>MGNIMSASFAPECTDLKTKYDSCFNEWYSEKFLKGKSVENECSKQWYAYTTCVNAALVKQGIKPALDEAREEAPFENGGKL[8x];>MGSSHHHHHHSQDPMVLLHKSTHIFPTDFASVSRAFFNRYPNPYSPHVLSIDTISRNVDQEGNLRTTRLLKKSGKLPTWVKPFLRGITETWIIEVSVVNPANSTMKTYTRNLDHTGIMKVEEYTTYQFDSATSSTIADSRVKFSSGFNMGIKSKVEDWSRTKFDENVKKSRMGMAFVIQKLEEA[8x]

Recently, Ups1, a yeast member of the conserved mitochondrial intermembrane space (IMS) proteins, was shown to mediate PA transfer between the mitochondrial OM and IM in cooperation with Mdm35. Mdm35, another conserved yeast IMS protein, is a binding partner of Ups proteins, and facilitate their import into mitochondria. Surprisingly, two distinct polypeptides of Ups1 and Mdm35 form a single compact domain, the Ups1 part of which corresponds to the START (StAR-related lipid-transfer) domain, likely functioning as a lipid-binding domain. Like other START domain-containing proteins, the Ups1–Mdm35 complex contains a deep pocket that can accommodate a lipid molecule and an Ω-loop likely functioning as a lid for the pocket.

Although we could not obtain good diffraction data of the Ups1–Mdm35 complex with POPA suitable for high-resolution structure determination, we successfully determined the crystal structure of the Ups1–Mdm35 complex with DLPA at 3.20 Å resolution by the molecular replacement method with the Ups1–Mdm35 apo-complex as a search model. The crystallographic asymmetric unit contained eight Ups1–Mdm35 molecules, and two of the eight Ups1–Mdm35 molecules contained a DLPA molecule in the pocket while clear electron density was not observed in the pocket of the remaining six Ups1–Mdm35 molecules. Structural comparison of the Ups1–Mdm35 complexes with and without a bound PA molecule shows the r.m.s. differences of 1.2 and 0.6 Å for 169 Cα atoms of Ups1 and 73 Cα atoms of Mdm35, respectively, indicating that no significant conformational change occurs in Ups1–Mdm35 on PA binding. Interestingly, some of the Ups1–Mdm35 molecules without clear electron density of DLPA in the crystallographic asymmetric unit had the Ω1 lid swung away from the pocket. The bound DLPA molecule is completely enclosed in the pocket of Ups1, with the phosphate head positioned at the bottom of the pocket and the acyl-chain tails oriented toward the entrance of the pocket, yet leaving some empty space in the pocket. At the bottom of the pocket, the positively charged side chains of Arg25 and Lys58 are close to the negatively charged phosphate group of DLPA, and side chains of Tyr26, His33 and Lys58 are within the distance that allows formation of hydrogen bonds with the phosphate oxygen atoms. The hydrophobic acyl-chain tails are in contact with hydrophobic side chains of Thr76, Ile78, Met104 and Val106 in the pocket. Besides, we found that the Ω1 lid could take an alternative open conformation that provides a wide space rendering the pocket entrance accessible to PA. Since the size of the entrance of the pocket is about 9 Å in diameter, which is too narrow to allow two acyl tails of PA to pass through freely, PA binding to the pocket may require opening of the entrance as well as a swing of the Ω1 lid away from the pocket entrance. The closed Ω1 lid may be important for preventing the bound PA molecules from slipping off the pocket, as well.> YEQDKTYKITVLHTNDHHGHFWRNEYGEYGLAAQKTLVDGIRKEVAAEGGSVLLLSGGDINTGVPESDLQDAEPDFRGMNLVGYDAMAIGNHEFDNPLTVLRQQEKWAKFPLLSANIYQKSTGERLFKPWALFKRQDLKIAVIGLTTDDTAKIGNPEYFTDIEFRKPADEAKLVIQELQQTEKPDIIIAATHMGHYDNGEHGSNAPGDVEMARALPAGSLAMIVGGHSQDPVCMAAENKKQVDYVPGTPCKPDQQNGIWIVQAHEWGKYVGRADFEFRNGEMKMVNYQLIPVNLKKKRVLYTPEIAENQQMISLLSPFQNK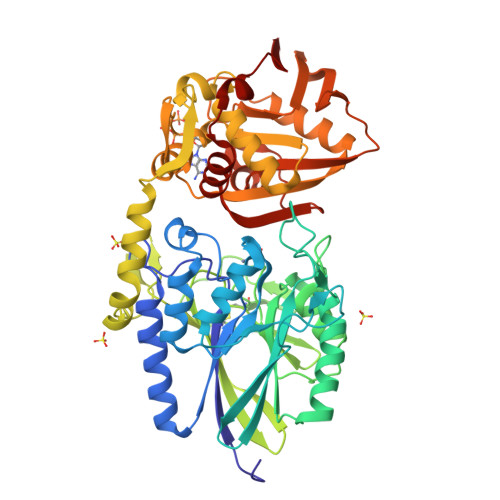GKAQLEVKIGETNGRLEGDRDKVRFVQTNMGRLILAAQMDRTGADFAVMSGGGIRDSIEAGDISYKNVLKVQPFGNVVVYADMTGKEVIDYLTAVAQMKPDSGAYPQFANVSFVAKDGKLNDLKIKGEPVDPAKTYRMATLNFNATGGDGYPRLDNKPGYVNTGFIDAEVLKAYIQKSSPLDVSVYEPKGEVSWQ> GSHMLSDEQMQIINSLVEAHHKTYDDSYSDFVRFRPPVREGPVTRSASRAASLHSLSDASSDSFNHSPESVDTKLNFSNLLMMYQDSGSPDSSEEDQQSRLSMLPHLADLVSYSIQKVIGFAKMIPGFRDLTAEDQIALLKSSAIEIIMLRSNQSFSLEDMSWSCGGPDFKYCINDVTKAGHTLEHLEPLVKFQVGLKKLKLHEEEHVLLMAICLLSPDRPGVQDHVRIEALQDRLCDVLQAYIRIQHPGGRLLYAKMIQKLADLRSLNEEHSKQYRSLSFQPEHSMQLTPLVLEVFG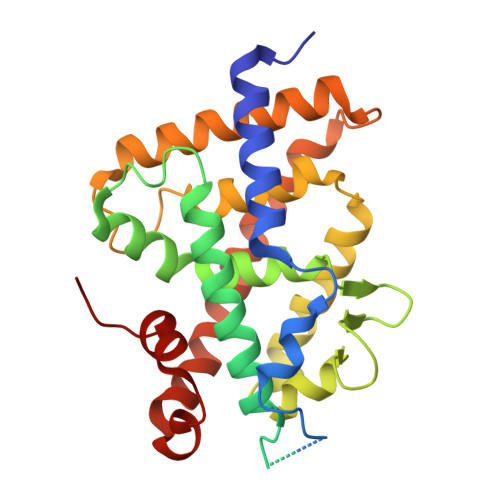SEVS> AAMEELQKSIGHKPEPTDEEWELIKTVTEAHVATNTQGS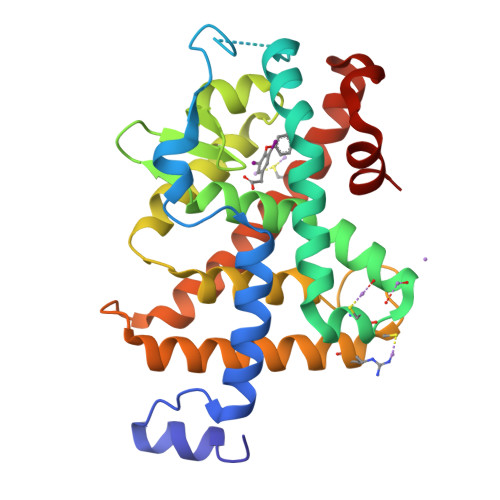HWKQKRKFLPEDIGQAPIVNAPEGGKVDLEAFSHFTKIITPAITRVVDFAKKLPMFCELPCEDQIILLKGCCMEIMSLRAAVRYDPESETLTLNGEMAVTRGQLKNGGLGVVSDAIFDLGMSLSSFNLDDTEVALLQAVLLMSSDRPGLACVERIEKYQDSFLLAFEHYINYRKHHVTHFWPKLLMKVTDLRMIGACHASRFLHMKVECPTELFPPLFLEVFED>MMKWSNKDGYPWSKIIHAEKFFDKVIQNDTRPGKWEWADVVSGLRDLDKDPRMNSERRYVAIVNEDVGLGETKGIGITPGLFCGCQLIHPGEEVTSHRHNSVALYFIVEGTGELEVEGEVYSYKPFDIMTCPAWSYHAWRATGDKDTLMYVIHDMALLAYMRALFWEEPKGSENIRHMVKGSTHTWSNTKAPEVSKTQAAKELLKQGE[4x]

5-Nitrosalicylate dioxygenase (EC 1.13.11.64; 5NSDO), isolated from the soil bacterium Bradyrhizobium sp. JS329, is an enzyme involved in the degradation of 5-nitroanthranilic acid, which is produced biologically for an unknown purpose by Streptomyces scabies and also industrially in the synthesis of nitroaromatic products and dyes. The degradation pathway is initiated by hydrolytic removal of the amino group catalyzed by an aminohydrolase to form 5-nitrosalicylate, which is then oxidized by 5NSDO, which cleaves the aromatic ring with the production of 4-nitro-6-oxohepta-2,4-dienedioic acid. 5NSDO is a nonheme iron(II)- and oxygen-dependent enzyme that belongs to the third class of ring-cleaving dioxygenases as it cleaves the aromatic ring of 5-nitrosalicylate, an ortho-hydroxy-substituted carboxylic acid. The enzyme also catalyzes the oxidation of 5-chlorosalicylate, while it is not active towards gentisate, salicylate, 5-hydroxyanthranilate, 4-nitrocatechol or 4-chlorocatechol.

The crystal structure of 5NSDO from Bradyrhizobium sp. was determined at 2.1 Å resolution by the molecular-replacement technique using a theoretical model predicted by AlphaFold. The asymmetric unit contains one tetramer. Each subunit of 5NSDO folds as a monocupin domain (residues 81–152) which consists of eight β-strands organized into two four-stranded antiparallel β-sheets that are a characteristic feature of this superfamily (β-barrel). The tetramer is mainly stabilized by the long flexible N-terminal region of each subunit, which makes interactions with all three of the other subunits. The quaternary structure is arranged in such a way that the active metal sites are oriented towards the external edge of the tetramer. Comparing the 5NSDO structure with those of closely related ring-cleaving dioxygenases of the same class, for example SDO and GDO, we found that the active-site residues are poorly conserved, as expected from the unusual activity exhibited by the enzyme, which accepts 5-chloro­salicylate and 5-nitrosalicylate as substrates but not gentisate and salicylate. Specifically, the residues which interact with the 5-OH group of gentisate (Asp174 and Trp104) are missing in 5NSDO, explaining the lack of activity of 5NSDO towards gentisate. Arg127, which is supposed to facilitate the deprotonation of the substrate in SDO, is substituted by Tyr104 in 5NSDO, likely due to the lower pK a of the substrate hydroxyl group compared with salicylate. Unfortunately, in all four 5NSDO subunits electron density for the side chain of Tyr58 was absent, so it was not included in the model.Here, the current status of the fully automated ambient-temperature beamline VMXi at Diamond Light Source is described, and a highly efficient pipeline from protein sample to final multi-crystal data analysis and structure determination is shown. The VMXi beamline and its associated PXF within the Research Complex at Harwell offer a highly automated pipeline where researchers provide a suitable protein sample that is used for robotic crystallization, monitoring and subsequent in situ data collection from crystals in crystallization plates or in thin-film sample delivery systems. Here we present illustrative examples of data measured using VMXi from a variety of proteins comprising both conventional crystallographic standards and ‘real world’ user samples. Routine RT data collection provides a useful capability that is highly relevant to studying protein dynamics and ligand binding without the complication of cryo-cooling.

As an example, here we show a project that focused on a range of nutrient-uptake proteins isolated from a marine cyano­bacteria (Synechococcus MITS9220). Once pure protein was available for a number of these proteins, they were put through crystallization screens en masse in the PXF, and subsequently potential crystallization hits were identified and analysed by data collection at VMXi. The overall fold of the two MITS9220_PhnD1 structures with phosphate is very similar, with a root mean squared deviation (RMSD) of 0.15 Å. The availability of the two structures in complex with phosphate provided an opportunity to directly compare the ligand binding site and understand if temperature bias potentially led to any differences in the ligand-binding interactions. Within the crystal structure of MITS9220_PhnD1 RT structure, the four phosphate oxygens are stabilized by ten direct hydrogen bonds with main-chain or side-chain atoms of Tyr44, Ser124, Thr125, Ser126, His156, Asp203 and Tyr204, as well as a water molecule buried deep within the cavity. Given the similarity of the 3D fold of the two MITS9220_PhnD1 structures, unsurprisingly, all four oxygen atoms of the phosphate moiety in the MITS9220_PhnD1 cryo-structure showed an identical hydrogen-bond network [Fig. 3(a)]. Thus, no temperature bias was introduced at the global or local scale for the MITS9220_PhnD1 protein. Even though the average B factors for the main/side chain and the solvent are higher for the RT MITS9220_PhnD1 structure compared with the cryo MITS9220_PhnD1 structure, overall, the two structures depict identical dynamic motion and flexibility trends.

> GPMQPRLKVGAIPDQNPERLNRLYGQLADELSDRLNVKVRYVPVSNYPAAVSAFRTGGLDLVWFGGLTGVQARLQTPGAQVLAQRDIDARFRSVFIANTSSGLQPISSINGLTSLRGKRFSFGSESSTSGRLMPQHFLAKAGVTPSQFSGGRAGFSGSHDATIAVVQSGAYEAGALNEQVWTSAVNDGRVNTEKVSVIWRTPEYVDYHWVVRPKLDQRFGKGFTTRLQKAILGLEPTTPRQVTILELFAAKRFIPVEASQYKPIEKVGRELGKIR>[2x]MKDFKLAKSKSHAIEETKPFSILLMGVDTGSEHRKSKWSGNSDSMILVTINPKTNKTTMTSLERDVLIKL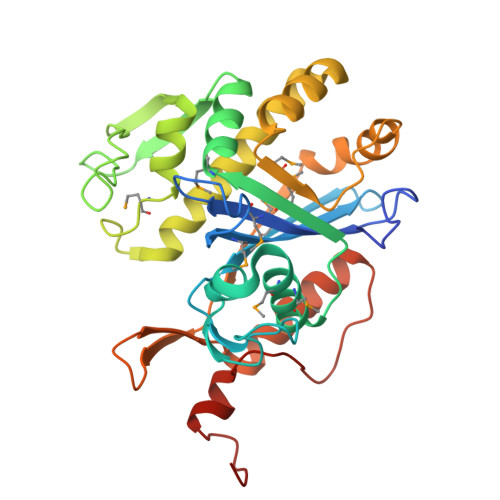SGPKNNGQTGVEAKLNAAYASGGAEMALMTVQDLLDINVDYFMQINMQGLVDLVNAVGGITVTNKFDFPISIAANEPEYKAVVEPGTHKINGEQALVYSRMRYDDPEGDYGRQKRQREVIQKVLKKILALNSISSYKKILSAVSNNMQTNIEISSKTIPNLLAYKDSLEHIKSYQLKGEDATLSDGGSYQILTKKHLLAVQNRIKKELDKKRSKTLKTSAILYEDYYGLEHHHHHH> QQFFFENDALGQSSTDFATNFLNLWDNNREQLLNLYSPQSQFSVSVDSTIPPSTVTDSDQTPAFGYYMSSSRNISKVSSEKSIQQRLSIGQESINSIFKTLPKTKHHLQEQPNEYSMETISYPQINGFVITLHGFFEETGKPELESNKKTGKNNYQKNRRYNHGYNSTSNNKLSKKSFDRTWVIVPMNNSVIIASDLLTVRAYSTGAWKTASIAIAQAAGS;> MNTNSNTMVMNDANQAQ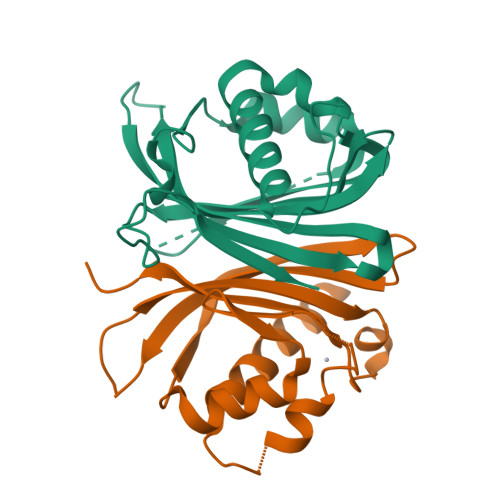ITATFTKKILAHLDDPDSNKLAQFVQLFNPNNCRIIFNATPFAQATVFLQMWQNQVVQTQHALTGVDYHAIPGSGTLICNVNCKVRFDESGRDKMGQDATVPIQPNNTGNRNRPNDMNKPRPLWGPYFGISLQLIIDDRIFRNDFNGVISGFNYNMVYKPEDSLLKI RAS is a major anticancer drug target which requires membrane localization to activate downstream signal transduction. Phosphodiesterase 6δ (PDE6D) has a beta-sandwich immunoglobulin fold which contains a hydrophobic pocket capable of binding to the farnesyl group. PDE6D binds to and sequesters the lipid of cytoplasmic RAS and has been proposed to deliver GTPase to recycling endosomes, which is followed by release mediated by the small G-protein Arf-like 2 (ARL2), allowing RAS to be trafficked back to the plasma membrane. The resultant lipid modification increases the affinity of RAS proteins toward membranes, where it is required for signal transduction. Here, we present a novel strategy for targeting RAS by stabilizing its interaction with the prenyl-binding protein PDE6D and disrupting its localization.

Two cocrystal structures with the fragments identified in the screen were successfully obtained: compound-1 in a ternary complex with PDE6D and WT KRAS peptide and compound-2 in complex with PDE6D alone. In the crystal structure of PDE6D:KRAS peptide:compound-1, the asymmetric unit contains two copies of the ternary complex. In each copy, the KRAS peptide is present in a unique conformation, a phenomenon which has not been previously observed. To our surprise, the fragment is located deep within the PDE6D cargo-binding pocket at the interface of KRAS and PDE6D, binding adjacent to the farnesyl group of KRAS. In one copy of the ternary complex, the compound is at 100% occupancy, while in the second ternary complex, it is modeled at 50% occupancy. With only 50% occupancy, several side chains within the PDE6D-binding pocket are in multiple conformations. In both instances, the fragment forms hydrogen bond interactions with the PDE6D R61 guanidine group, Q78 side chain, and carbonyl oxygen of the W105 peptide bond. Compound-1 showed no competition with KRAS in either experiment; however, compound-2 did show competition with the KRAS WT peptide. Overlay of the two complexes containing compound-1 and compound-2 shows that these fragments are within close proximity to each other with a distance of 4.8 Å between the two closest atoms.

>MSAKDERAREILRGFKLNWMNLRDAETGKILWQGTEDLSVPGVEHEARVPKKILKCKAVSRELNFSSTEQMEKFRLEQKVYFKGQCLEEWFFEFGFVIPNSTNTWQSLIEAAPESQMMPASVLTGNVIIETKFFDDDLLVSTSRVRLFYV[2x];>DGKKKKKKSKTKC[2x]> MSKIESALQAAQPGLSRLRGGAGGMGYRAATTQAEQPRSSLLDTIGRFAKAGADMYTAKEQRARDLADERSNEIIRKLT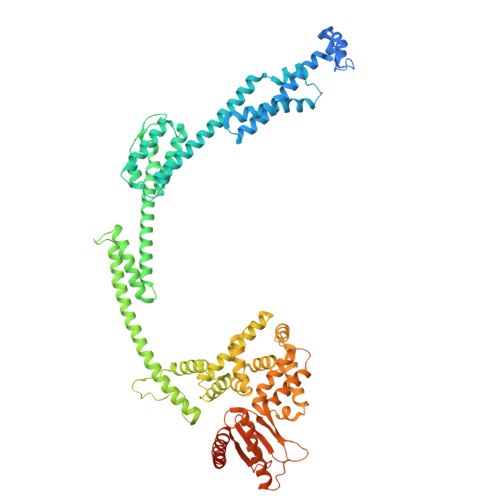PEQRREALNNGTLLYQDDPYAMEALRVKTGRNAAYLVDDDVMQKIKEGVFRTREEMEEYRHSRLQEGAKVYAEQFGIDPEDVDYQRGFNGDITERNISLYGAHDNFLSQQAQKGAIMNSRVELNGVLQDPDMLRRPDSADFFEKYIDNGLVTGAIPSDAQATQLISQAFSDASSRAGGADFLMRVGDKKVTLNGATTTYRELIGEEQWNALMVTAQRSQFETDAKLNEQYRLKINSALNQEDPRTAWEMLQGIKAELDKVQPDEQMTPQREWLISAQEQVQNQMNAWTKAQAKALDDSMKSMNKLDVIDKQFQKRINGEWVSTDFKDMPVNENTGEFKHSDMVNYANKKLAEIDSMDIPDGAKDAMKLKYLQADSKDGAFRTAIGTMVTDAGQEWSAAVINGKLPERTPAMDALRRIRNADPQLIAALYPDQAELFLTMDMMDKQGIDPQVILDADRLTVKRSKEQRFEDDKAFESALNASKAPEIARMPASLRESARKIYDSVKYRSGNESMAMEQMTKFLKESTYTFTGDDVDGDTVGVIPKNMMQVNSDPKSWEQGRDILEEARKGIIASNPWITNKQLTMYSQGDSIYLMDTTGQVRVRYDKELLSKVWSENQKKLEEKAREKALADVNKRAPIVAATKAREAAAKRVREKRKQTPKFIYGRKE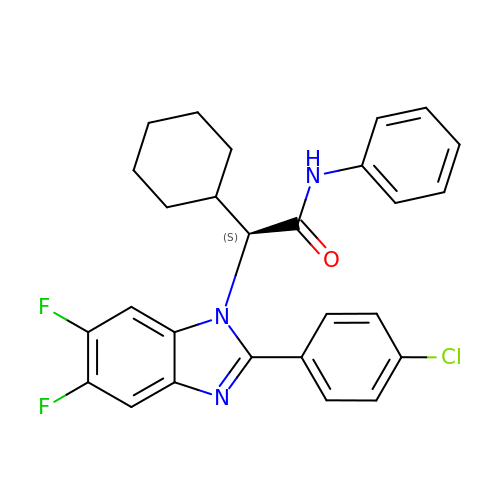(2S)-2-[2-(4-chlorophenyl)-5,6-difluoro-1H-benzimidazol-1-yl]-2-cyclohexyl-N-phenylacetamide | C27 H24 Cl F2 N3 O | ARWUUCFDBAFWCD-VWLOTQADSA-N> GVGISTGTFNNQTEFKFLENGWVEITANSSRLVHLNMPESENYRRVVVNNMDKTAVNGNMALDDIHAQIVTPWSLVDANAWGVWFNPGDWQLIVNTMSELHLVSFEQEIFNVVLKTVSESATQPPTKVYNNDLTASLMVALDSNNTMPFTPAAMRSETLGFYPWKPTIPTPWRYYFQWDRTLIPSHTGTSGTPTNIYHGTDPDDVQFYTIENSVPVHLLRTGDEFATGTFFFDCKPCRLTHTWQTNRALGLPPFLNSLPQSEGATNFGDIGVQQDKRRGVTQMGNTNYITEATIMRPAEVGYSAPYYSFEASTQGPFKTPIAAGRGGAQTDENQAADGNPRYAFGRQHGQKTTTTGETPERFTYIAHQDTGRYPEGDWIQNINFNLPVTNDNVLLPTDPIGGKTGINYTNIFNTYGPLTALNNVPPVYPNGQIWDKEFDTDLKPRLHVNAPFVCQNNCPGQLFVKVAPNLTNEYDPDASANMSRIVTYSDFWWKGKLVFKAKLRASHTWNPIQQMSINVDNQFNYVPSNIGGMK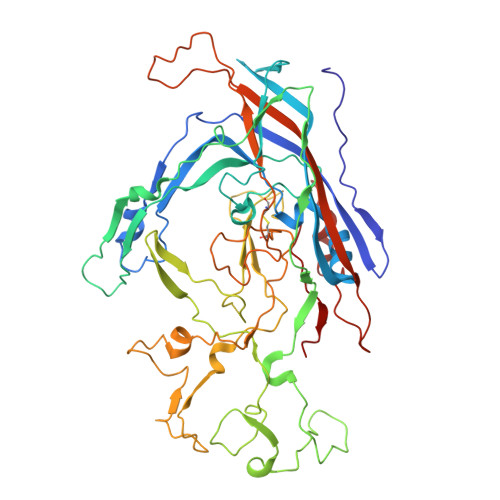IVYEKSQLAPRKLY>[4x]GSMGVEEVVNNKAKRLIDIYHAAVKELIQNEELIDLIDKHNVDYSVIESIENLPNLADINVKDDIDDVLSEIIKKKEVKIGALKNKNWGIIGNYEQNPPVGFWPDVMYIIWETISKHIFNDEDAINIAYNYYDNVFV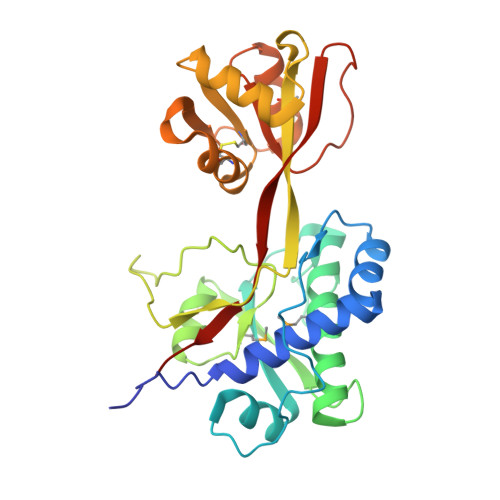ALNDKDIHMTDNYFLSNSRLVDQSGNNLPKLTSGLPIIKHSNKIMILKEYNINNLEDLKSYISKNEGLKIACLTEANCNALKNIFLDKVTYDYKSFSSYIDLSKSVLSKSHIIGVISGIPFNFNEHKINVFDSFLKTGHSAYFKAAA> MKIFSESHKTVFVVDHCPYMAESCRQHVEFDMLVKNRTQGIIPLAPISKSLWTCSVESSMEYCRIMYDIFPFKKLVNFIVSDSGAHVLNSWTQEDQNLQELMAALAAVGPPNPRADPECCSILHGLVAAVETLCKITEYQHEARTLLMENAERVGNRGRIICITNAKSDSHVRMLEDCVQETIHEHNKLAANSDHLMQIQKCELVLIHTYPVGEDSLVSDRSKKELSPVLTSEVHSVRAGRHLATKLNILVQQHFDLASTTITNIPMKEEQHANTSANYDVELLHHKDAHVDFLKSGDSHLGGGSREGSFKETITLKWCTPRTNNIELHYCTGAYRISPVDVNSRPSSCLTNFLLNGRSVLLEQPRKSGSKVISHMLSSHGGEIFLHVLSSSRSILEDPPSISEGCGGRVTDYRITDFGEFMRENRLTPFLDPRYKIDGSLEVPLERAKDQLEKHTRYWPMIISQTTIFNMQAVVPLASVIVKESLTEEDVLNCQKTIYNLVDMERKNDPLPI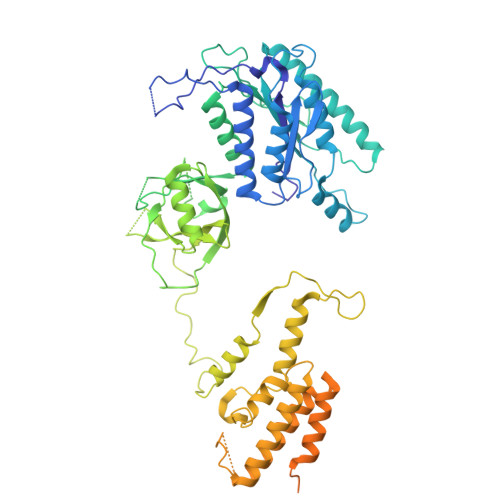STVGTRGKGPKRDEQYRIMWNELETLVRAHINNSEKHQRVLECLMACRSKPPEEEERKKRGRKREDKEDKSEKAVKDYEQEKSWQDSERLKGILERGKEELAEAEIIKDSPDSPEPPNKKPLVEMDETPQVEKSKGPVSLLSLWSNRINTANSRKHQEFAGRLNSVNNRAELYQHLKEENGMETTENGKASRQ A crucial role in this process is played by centromeres, specialized chromatin domains whose defining mark in almost all known eukaryotes is the enrichment of centromeric protein A (CENP-A, also known as CenH3), which replaces histone H3 in nucleosomes. The primary function of centromeres is to provide a platform for the assembly of macromolecular complexes known as kinetochores, whose task in turn is the physical capture of microtubules of the mitotic spindle. In vitro, these interact specifically and selectively with two CCAN components, CENP-C and CENP-N. Binding of these proteins to CENP-A nucleosomes has been shown to require two regions where the CENP-A sequence diverges significantly from that of histone H3, the L1 loop and the C-terminal tail. In conclusion, the structure of CENP-N contains an N-terminal Pyrin domain, a central CLN-HD, and a C-terminal CENP-L dimerization domain, while CENP-L contains an N-terminal CLN-HD, interrupted immediately before the C-terminal helix by an insertion that contains a region required for CENP-N dimerization.

We obtained well diffracting crystals of the CENP-N1-235 construct and determined its crystal structure at 2.8 Å resolution. CENP-N1-235 consists of two closely juxtaposed domains that interact through an extended interface to form a single structural unit. The first domain (residues 1–77) consists of a five-helix bundle, whereas the second domain (residues 78–212, cyan in Figure 1A) consists of a six-stranded anti-parallel β-sheet sandwiched between α-helices. There is no clear density beyond residue ~210, indicating that the structure is disordered after this point. Fold-recognition by DALI identified similarity of the first domain to PYRIN domains (PYDs; a superposition is shown in Figure 2—figure supplement 1A–B). Besides identifying the N-terminal domain of CENP-N1-235 as a PYRIN domain, DALI also identified an unanticipated structural homology of the second domain of CENP-N1-235 with the N-terminal domain of Iml3CENP-L. We therefore refer to these domains of CENP-N and CENP-L as CLN-HD (for CENP-L and CENP-N homology domain). Monomers A and B in the asymmetric unit are quite similar except for a minor hinge-bending between the two subdomains of each monomer, and except for loops 137–142 and 164–174. Our study did not identify a clear structural basis for this phenomenon, as we failed to identify significant conformational changes in CENP-N in isolation (crystal structure) compared to its complex with CENP-ANCP.

>[2x]MDETVAEFIKRTILKIPMNELTTILKAWDFLSENQLQTVNFRQRKESVVQHLIHLCEEKRASISDAALLDIIYMQFHQHQKVWDVFQMSKGPGEDVDLFDMKQFKNSFKKILQRALKNVTVSFRETEENAVWIRIAWGTQYTKPNQYKPTYVVYYSQTPYAFTSSSMLRRNTPLLGQALTIASKHHQIVKMDLRSRYLDSLKAIVFKQYNQTFHHHHHH> HCEGX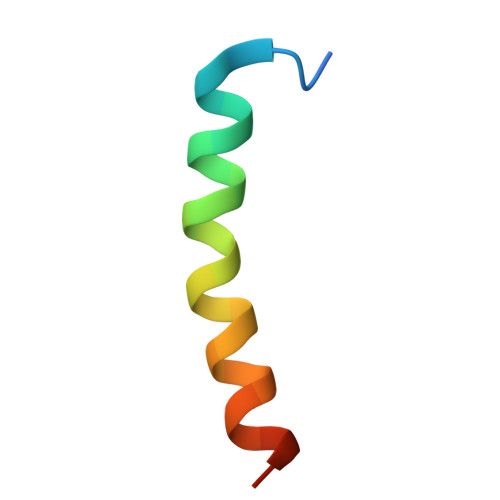FTSDVSSYLEGQAAKEFIAWLVKGRG> MKKETIFSEVETANSKQLAVLKANFPQCFDKNGAFIQEKLLEIIRASEVELSKESYSLNWLGKSYARLLANLPPKTLLAEDKTHNQQEENKNSQHLLIKGDNLEVLKHMVNAYAEKVKMIYIDPPYNTGKDGFVYNDDRKFTPEQLSELAGIDLDEAKRILEFTTKGSSSHSAWLTFIYPRLYIARELMREDGTIFISIDHNEFSQLKLVCDEIFGEQNHVGDLVWKNATDNNPSNIAVEHEYIIVYTKNKEQLISEWKSNISDVKNLLVNIGEEFASKYTGNELQEKYTQWFREHRSELWPLDRYKYIDKDGIYTGSQSVHNPGKEGYRYDIIHPKTKKPCKQPLMGYRFPLDTMDRLLSEEKIIFGDDENKIIELKVYAKDYKQKLSSVIHLDGRVATNELKELFPEMTQPFTNAKTIKLVEDLISFACDGEGIVLDFFAGSGTTAHTVFNLNNKNKTSYQFITVQLDEPTKDKSDAMKHGYNTIFDLTKERLIRASKKNRDQGFKVYQLMPDFRAKDESELTLSNHTFFDDVVLTPEQYDTLLTTWCLYDGSLLTTPIEDVDLGGYKAHLCDGRLYLIAPNFTSEALKALLQKVDSDKDFAPNKVVFYGSNFESAKQMELNEALKSYANKKSI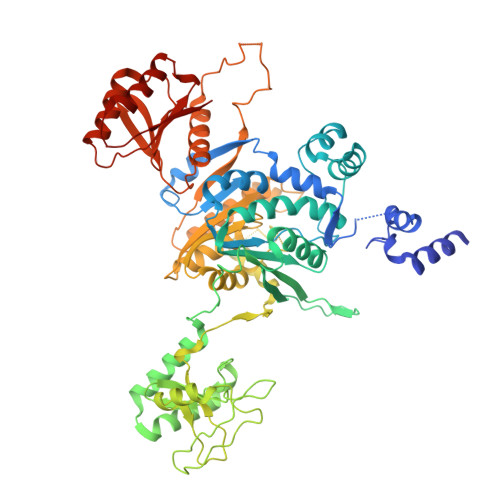ELDLVVRN> MSGKIVRAPSNWTTPHKKMLKEDEDQELIAFDKLLSWVSETGVGTEEQAKIVFKKINAYFYLRCLYPVLPRDPKSMKIFQLNLHFLILGYIIDDAIEKYNENEMKELIAGYNLLQSQVSETFPNFPSIFEMKQLLGNMKNDFSKSAITTMFDYVNKTTLILLEEGEIAEHNVLNYRKRLSNAVAVYFDALLSKTKTGCEISDGAMLWRRCFDALAIAVYMLTEVFSKTLVKNHTLPVSEFYKFYLLSILFCVVINDLHSYERDKLDDTDSVVKVWFKEGSVANMEAATSKVSKILDAIIQQMYLFVEEGKARHPELSEWFERIAYMTVGWIYIHKTVVPRYVSSPFQIEVVE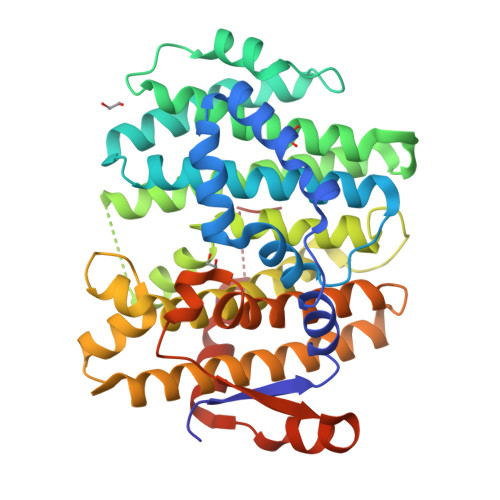IHENMISNWLLKKDAYGQRVVQQFLKNLNDPQKKNIMLYDE>[4x]MALHHHHHHGVTGELRRRADGIWQRILAHPFVAELYAGTLPMEKFKYYLLQDYNYLVNFAKALSLAASRAPSVDLMKTALELAYGTVTGEMANYEALLK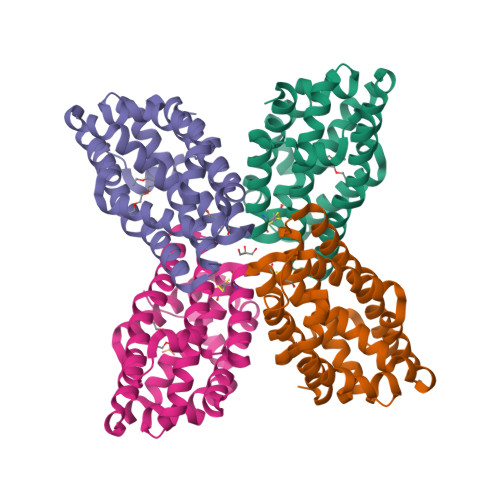EVGLSLRDAAEAEPNRVNVSYMAYLKSTCALEGFYQCMAALLPCFWSYAEIAERHGGKLRENPVHVYKKWASVYLSPEYRGLVERLRAVLDSSGLSAEELWPYFKEASLYELEFWQAAYEGH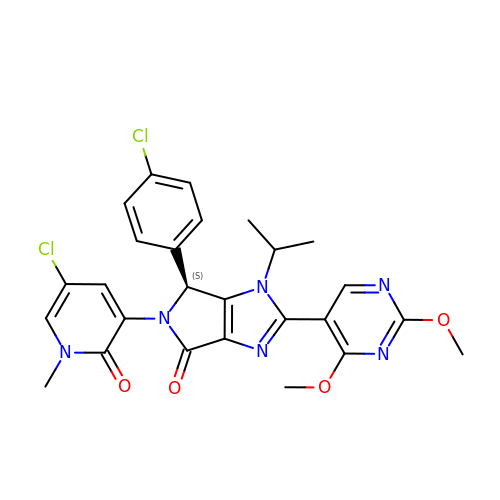(4~{S})-5-(5-chloranyl-1-methyl-2-oxidanylidene-pyridin-3-yl)-4-(4-chlorophenyl)-2-(2,4-dimethoxypyrimidin-5-yl)-3-propan-2-yl-4~{H}-pyrrolo[3,4-d]imidazol-6-one | C26 H24 Cl2 N6 O4 | AGBSXNCBIWWLHD-FQEVSTJZSA-N> MGSMPKTLRQKLLLALIA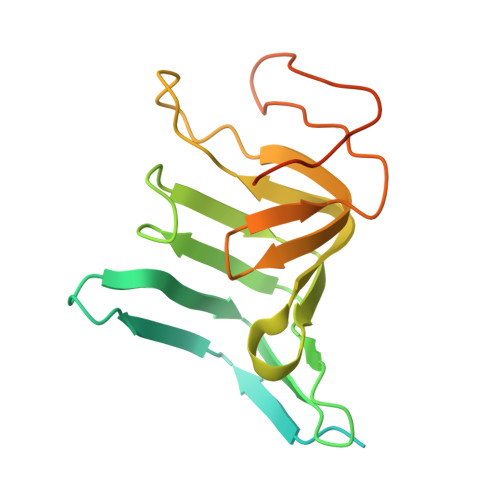LLLIVAGYYWNVGLELFNEQPTRPGQDNTIDYYAENAHSLQYQEDGSLDYEMTAVKLEHQKATDITFVTTPDLLLFRGNVQPWHIQSARAEVGPKGKEVELIDDVRVARTDAKGQPSILTTTRLTVFPDKNYAQTEQAVKIDAANGVTTAVGMKAYLKDSRMHLLSNVRGQHEVR HPRT is a purine salvage enzyme that converts purine bases and PRPP to GMP and IMP, which are precursors of the essential nucleotide GTP. HPRT activity was previously found to be inhibited by (p)ppGpp in several bacteria including Bacillus subtilis. To examine the molecular determinants underlying (p)ppGpp regulation of HPRT, we turned to Hpt-1 from the pathogenic bacterium B. anthracis, which pppGpp competitively inhibits similarly to B. subtilis HPRT. We crystallized Hpt-1 with and without ppGpp, and for comparison, we also crystallized Hpt-1 with its two substrates, PRPP and the non-reactive guanine analog 9-deazaguanine.

The HPRT-substrates structure diffracted to 1.64 Å containing two molecules in the asymmetric unit, and PRPP and 9-deazaguanine were coordinated by two Mg2+ ions with each monomer. The purine ring of ppGpp overlaps with the purine base substrate, and the two phosphate arms of ppGpp and PRPP both spread across the active site between loop I and loop III. We noticed a significant difference between the ppGpp- and substrates-bound tertiary structures in the conformation of a flexible loop. This loop, also called loop II, is common to all HPRTs and covers the active site during catalysis. In the substrates-bound state, loop II is instead shifted ≈4 Å toward the active site from its position in the dimer-dimer interface. Loop II also pulls its flanking dimer interface components β3 and α3 toward the active site. While crystal contacts likely prevent loop II from completely moving over the active site, PISA analysis predicts that these changes abolish the dimer-dimer interaction. Taken together, these data reveal that HPRT binds PRPP as catalytically active dimers, whereas (p)ppGpp maintains HPRT as tetramers.

>[2x]SNAMMNQDIEKVLISEEQIQEKVLELGAIIAEDYKNTVPLAIGVLKGAMPFMADLLKRTDTYLEMDFMAVSSYGHSTVSTGEVKILKDLDTSVEGRDILIVEDIIDSGLTLSYLVDLFKYRKAKSVKIVTLLDKPTGRKVDLKADYVGFTVPHEFVVGYGLDYKEQYRNLPYVGVLKPSVYSN> HLNYRQKGVIDVFLHAWKGYRKFAWGHDELKPVSRSFSEWFGLG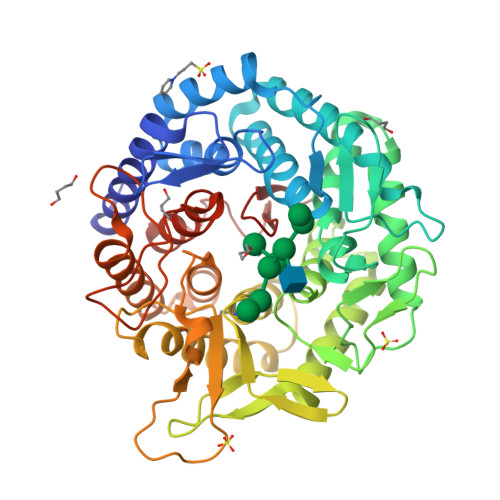LTLIDALDTMWILGLRKEFEEARKWVSKKLHFEKDVDVNLFESTIRILGGLLSAYHLSGDSLFLRKAEDFGNRLMPAFRTPSKIPYSDVNIGTGVAHPPRWTSDSTVAEVTSIQLEFRELSRLTGDKKFQEAVEKVTQHIHGLSGKKDGLVPMFINTHSGLFTHLGVFTLGARADSYYEYLLKQWIQGGKQETQLLEDYVEAIEGVRTHLLRHSEPSKLTFVGELAHGRFSAKMDHLVCFLPGTLALGVYHGLPASHMELAQELMETCYQMNRQMETGLSPEIVHFNLYPQPGRRDVEVKPADRHNLLRPETVESLFYLYRVTGDRKYQDWGWEILQSFSRFTRVPSGGYSSINNVQDPQKPEPRDKMESFFLGETLKYLFLLFSDDPNLLSLDAYVFNTEAHPLPIW> VTVTVNKNPSHTVPSTLYGLMFEDINHSGDGGLYAELLQNRAFQQVTPNTAAALAAWHPISNAKLAVIQDPSPVSNALPNSLQFSVPSGSSGRVGFTNEGFWGIKVDSTWTYKASLFFRFPTSSSFSGALTVGLQTNAGRVLAQNSTQIRGTTTKWTQINLELHPTASAPDVSNSFFVTIDGAAGAGQTINFAMFSLFPPTFKNRPNGLRADIAETLAEMGPSFFRFPGGNNLEGQTTATRWQWNATVGSLLDRPGRVGDWGYVNTDGLGLLEYLQFFEDTGMEPIMAVWAGYSLGGTSLAENQLAPYIQQAIDQINFVIGDPAKSAPAALRASLGHPEPFTLRFVEVGNEDFFAAGSYPYRWHDFVTALQAQFPQIRFIATTNAWNPVLSPVPQSYDVHVYQTPTWFYQNAFYYDGFQRNGTTYFEGEYAAISTNANDLFGTVADGRLAFPTVQSATGEAAFMTGLERNSDIVFAASYAPLLQHVNSTQWTPDLVSYDAGSVIKSTSFFAQKLFALNKGDQYLPSTLPTNGGTLHWSITRASSSGKTFIKIANAGSSAQSLTFQLTQFNSVSSTGTLQVLTGPETASNTPEAPQAIVPKTSTIGTGKTFTYNAPAFSVSVITVTTN

α-l-Arabinofuranosidases from glycoside hydrolase family 51 use a stereochemically retaining hydrolytic mechanism to liberate nonreducing terminal α-l-arabinofuranose residues from plant polysaccharides such as arabinoxylan and arabinan. Here, the crystallization and structural characterization of MgGH51, an industrially relevant GH51 α-l-arabinofuranosidase cloned from Meripilus giganteus, are reported. As in other GH51 enzymes, the N- and C-termini of the sequence are found in the 12-stranded β-sandwich domain, but unlike bacterial GH51 enzymes MgGH51 has a 169-residue ten-stranded β-sandwich domain inserted following the 36-residue N-terminal strand.

Using this chemical biology approach, we aimed to determine the structure of a fungal GH51 enzyme, identify its key catalytic residues and compare the catalytic sites and mechanisms of fungal and bacterial GH51 enzymes. To this end, we have crystallized MgGH51 and solved its structure in the unliganded state and in complex with l-arabinose, AraDNJ, α-l-AraAZI and α-l-AraCS. Clear density was present for the primary amine or sulfate group on C6 resulting from the ring-opening addition reaction. While the steric bulk of the sulfate group of α-l-AraCS caused some rearrangement of the active site, the addition of α-l-AraAZI to Glu429, leaving a primary amine in place of the sulfate, caused no apparent changes to the protein structure relative to the unliganded enzyme, suggesting that this structure is a good mimic for the natural glycosyl-enzyme intermediate. Crystal soaks with arabinose, 1,4-dideoxy-1,4-imino-l-arabinitol and two cyclophellitol-derived arabinose mimics reveal a conserved catalytic site and conformational itinerary between fungal and bacterial GH51 α-l-arabino­furanosidases.> MAL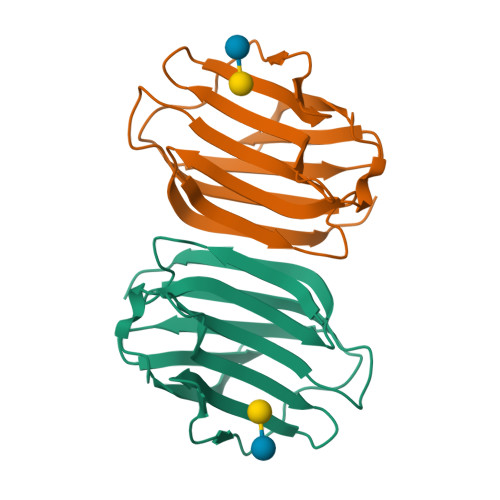RFEALYPEGMCPGWSVVVKGKTSSNTSMFEINFLSHPGDQIAFHFNPRFASSRIVCNSFLANHWGKEEVNKTFPFEAKEPFQVEIYSDQDYFHIFIDENKILQYKHRQKQLSSITKLQILNDIEISSVEITKRGLY>GAMGDEKIMETIASELKAIGKELEDQKKEENIQIAKIAKEKFDFLSTFKVGPYDLIDEDIQMKIKRTLYSSLDYKKENIEKLKEILEILKKNSEHYNIIGRLIYHISWGIQFQIEQNLELIQNGVEN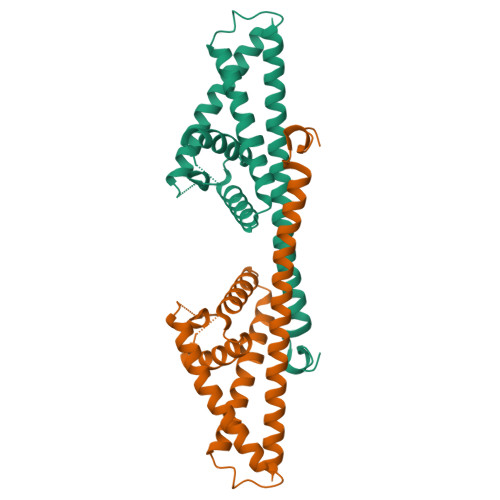LSQEESKSLLMQIKSNLEIKQRLKKTLNETLKVYNQNTQDNEKILAEHFNKYYKDFDTLKPAFY[2x]>IVCHTTATIPSSAVTCPPGENLCYRKMWCDAFCS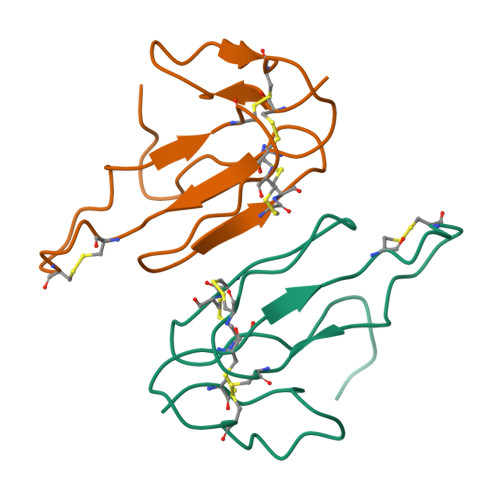SRGKVVELGCAATCPSKKPYEEVTCCSTDKCNHPPKRQPG[2x]> DHNTEEMENSADRVTTQTAGNTAINTQSSLGVLCAYVEDPTKSDPPSSSTDQPTTTFTAIDRWYTGRLNSWTKA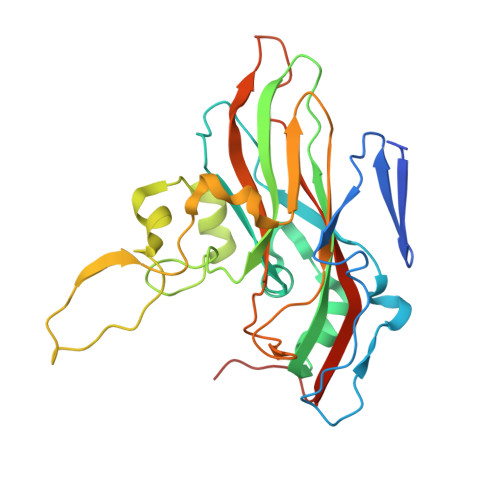VKTFSFQAVPLPGAFLSRQGGLNGGAFTATLHRHFLMKCGWQVQVQCNLTQFHQGALLVAMVPETTLDVKPDGKAKSLQELNEEQWVEMSDDYRTGKNMPFQSLGTYYRPPNWTWGPNFINPYQVTVFPHQILNARTSTSVDINVPYIGETPTQSSETQNSWTLLVMVLVPLDYKEGATTDPEITFSVRPTSPYFNGLRNRYTAGTDEEQ>[10x]MSLLSDLINLNLSDTTEKVIAEYIWIGGSGMDLRSKARTLPGPVSDPSKLPKWNYDGSSTGQAPGEDSEVIIYPQAIF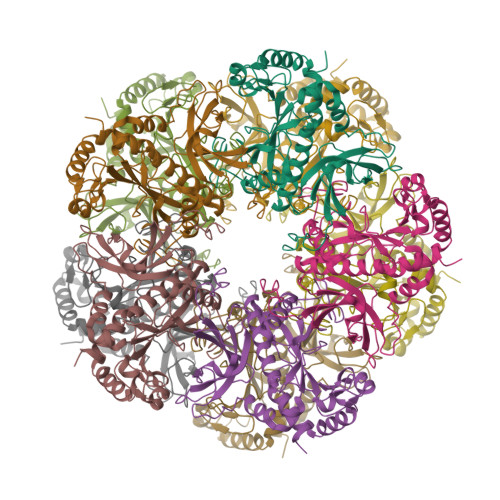RDPFRRGNNILVICDTYTPAGEPIPTNKRHDAAKVFSHPDVVAEETWYGIEQEYTLLQKDIQWPLGWPVGGFPGPQGPYYCGVGADKAFGRDIVDAHYKACLYAGINISGINGEVMPGQWEFQVGPSVGISAGDEVWAARYILERITEIAGVVVSFDPKPIQGDWNGAGAHTNYSTKSMRNDGGYEVIKTAIEKLGKRHKEHIAAYGEGNERRLTGRHETADINTFLWGVANRGASVRVGRDTEKAGKGYFEDRRPASNMDPYVVTSMIADTTILWKP> MPTPFLALPLIAEGQAGQHVTHNEALDMIDALAPRVVLSDSLATPPPAPPDRSAWIVPPGGSGFGGAGPGQIALRLGGVWHAITPAQGARWRVLDRGAAVIWSGTSWRPADVSGALGSTLGLATIE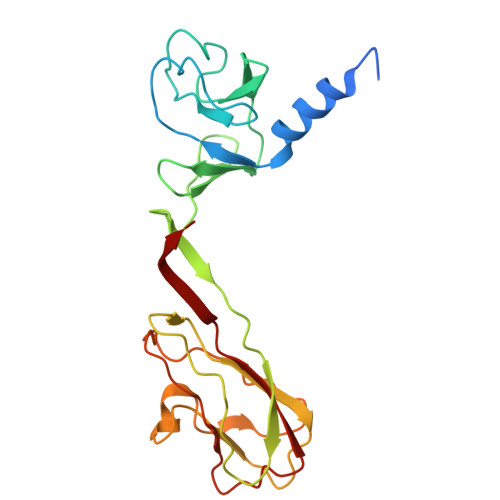ATVTATGPSVTAPALIPPRAIVLGVTSWTVQAVTGATSYRVGVPGEPDKFGASLGAAPGSSNIGVVGPFATYAPTDVVVTAEGADFTGGTIGLAASVILPGAPV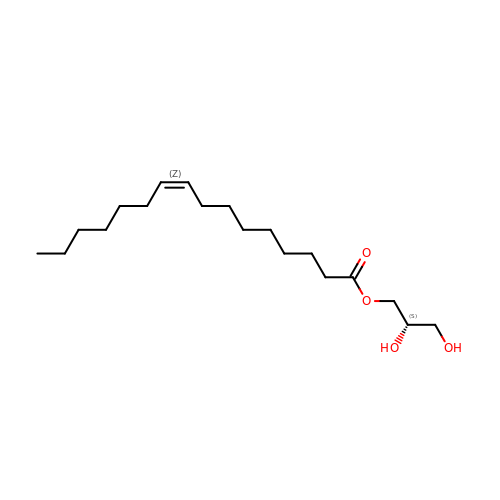(2S)-2,3-dihydroxypropyl (9Z)-hexadec-9-enoate | C19 H36 O4 | KVYUBFKSKZWZSV-ZEVQVBBLSA-N>[3x]MNSPVDAPKWPRQIPYIIASEACERFSFYGMRNILTPFLMTALLLSIPEELRGAVAKDVFHSFVIGVYFFPLLGGWIADRFFGKYNTILWLSLIYCVGHAFLAIFEHSVQGFYTGLFLIALGSGGIKPLVSSFMGDQFDQSNKSLAQKAFDMFYFTINFGSFFASLSMPLLLKNFGAAVAFGIPGVLMFVATVFFWLGRKRYIHMPPEPKDPHGFLPVIRSALLTKVEGKGNIGLVLALIGGVSAAYALVNIPTLGIVAGLCCAMVLVMGFVGAGASLQLERARKSHPDAAVDGVRSVLRILVLFALVTPFWSLFDQKASTWILQANDMVKPQWFEPAMMQALNPLLVMLLIPFNNFVLYPAIERMGVKLTALRKMGAGIAITGLSWIVVGTIQLMMDGGSALSIFWQILPYALLTFGEVLVSATGLEFAYSQAPKAMKGTIMSFWTLSVTVGNLW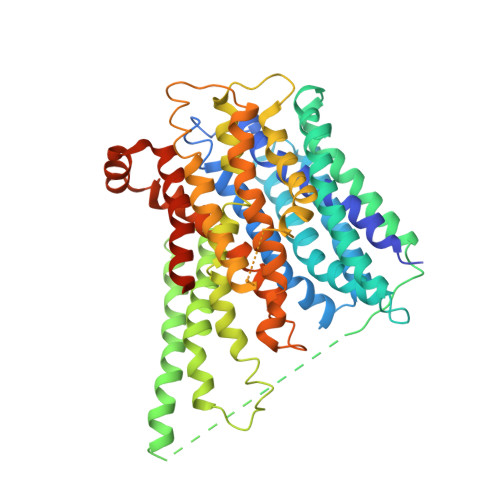VLLANVSVKSPTVTEQIVQTGMSVTAFQMFFFAGFAILAAIVFALYARSYQMQDHYRQATGSENLYFQ>[4x]MDMGISGKVAVITGSSSGIGLAIAEGFAKEGAHIVLVARQVDRLHEAARSLKEKFGVRVLEVAVDVATPEGVDAVVESVRSSFGGA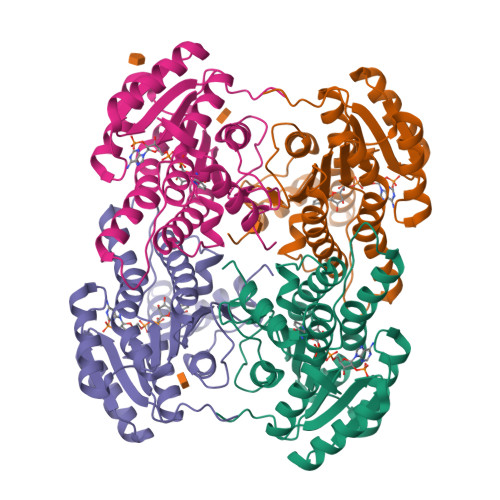DILVNNAGTGSNETIMEAADEKWQFYWELLVMAAVRLARGLVPGMRARGGGAIIHNASICAVQPLWYEPIYNVTKAALMMFSKTLATEVIKDNIRVNCINPGLILTPDWIKTAKELTKDNGGDWKGYLQSVADEHAPIKRFASPEELANFFVFLCSERATYSVGSAYFVDGGMLKTL> ADPQGVYAPAQAQIVHAGQACVVKEDNISERVYTIREGDTLMLQCLVTGHPRPQVRWTKTA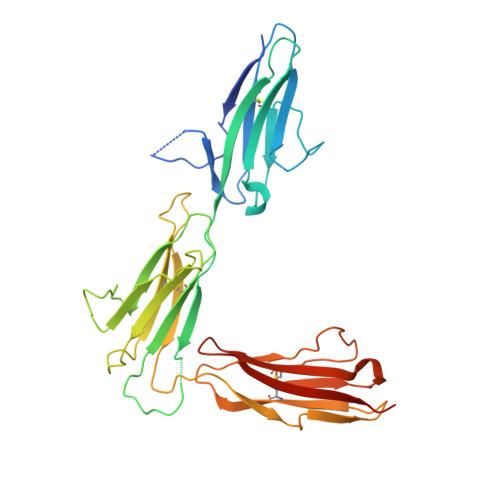GSASDKFQETSVFNETLRIERIARTQGGRYYCKAENGVGVPAIKSIRVDVQYLDEPMLTVHQTVSDVRGNFYQEKTVFLRCTVNSNPPARFIWKRGSDTLSHSQDNGVDIYEPLYTQGETKVLKLKNLRPQDYASYTCQVSVRNVCGIPDKAITFRLTNTTAPPALKLSVNETLVVNPGENVTVQCLLTGGDPLPQLQWSHGPGPLPLGALAQGGTLSIPSVQARDSGYYNCTATNNVGNPAKKTVNLLVRSMKLVPR> RSYGPVFEEQPAHTLFPEGSAEEKVTLTCRARANPPATYRWKMNGTELKMGPDSRYRLVAGDLVISNPVKAKDAGSYQCVATNARGTVVSREASLRFGFLQEFSAEERDPVKITEGWGVMFTCSPPPHYPALSYRWLLNEFPNFIPADGRRFVSQTTGNLYIAKTEASDLGNYSCFATSHIDFITKSVFSKFSQLSLAAEDARQYAPSIKAKFPADTYALTGQMVTLECFAFGNPVPQIKWRKLDGSQ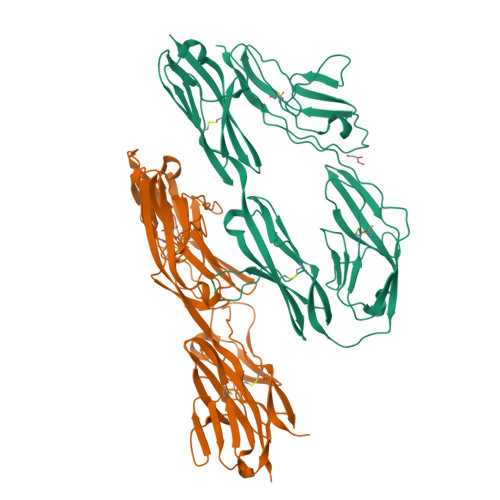TSKWLSSEPLLHIQNVDFEDEGTYECEAENIKGRDTYQGRIIIHAQPDWLDVITDTEADIGSDLRWSCVASGKPRPAVRWLRDGQPLASQNRIEVSGGELRFSKLVLEDSGMYQCVAENKHGTVYASAELTVQA>SITENTSWNKEFSAEAVNGVFVLCKSSSKSCATNDLARASKEYLPASTFKIPNAIIGLETGVIKNEHQVFKWDGKPRAMKQWERDLTLRGAIQVSAVPVFQQIAREVGEVRMQKYLKKFSYGNQNISGGIDKFWLEGQLRISAVNQVEFLESL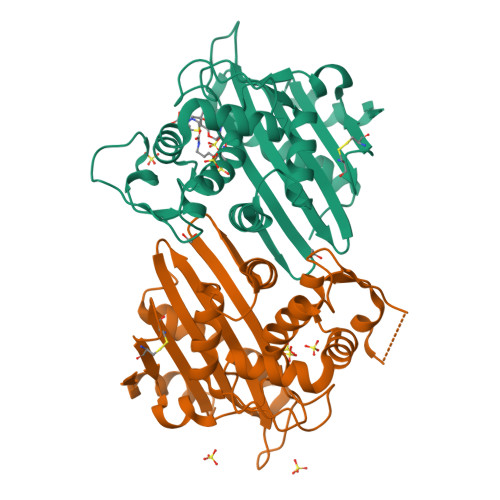YLNKLSASKENQLIVKEALVTEAAPEYLVHSKTGFSGVGTESNPGVAWWVGWVEKETEVYFFAFNMDIDNESKLPLRKSIPTKIMESEGIIGG[4x]> MKVQYCDSLVIGGGLAGLRAAVATQQKGLSTIVLSLIPVKRSHSAAAQGGMQASLGNSKMSDGDNEDLHFMDTVKGSDW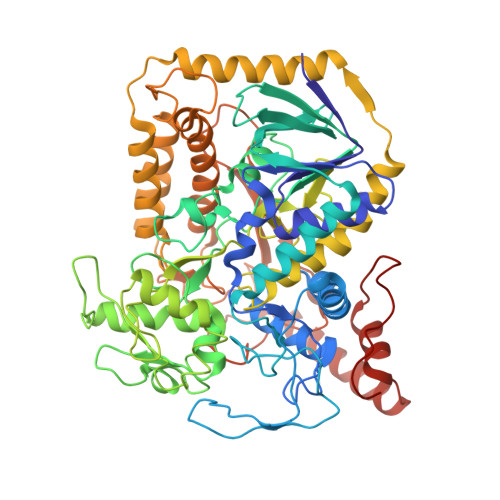GCDQKVARMFVNTAPKAIRELAAWGVPWTRIHKGDRMAIINAQKTTITEEDFRHGLIHSRDFGGTKKWRTCYTADATGHTMLFAVANECLKLGVSIQDRKEAIALIHQDGKCYGAVVRDLVTGDIIAYVAKGTLIATGGYGRIYKNTTNAVVCEGTGTAIALETGIAQLGNMEAVQFHPTPLFPSGILLTEGCRGDGGILRDVDGHRFMPDYEPEKKELASRDVVSRRMIEHIRKGKGVQSPYGQHLWLDISILGRKHIETNLRDVQEICEYFAGIDPAEKWAPVLPMQHYSMGGIRTDYRGEAKLKGLFSAGEAACWDMHGFNRLGGNSVSEAVVAGMIVGEYFAEHCANTQVDLETKTLEKFVKGQEAYMKSLVESKGTEDVFKIKNRMKDVMDDNVGIFRDGPHLEKAVKELEELYKKSKNVGIKNKRLHANPELEEAYRVPMMLKVALCVAKGALDRTESRGAHNREDYPKRDDINWLNRTLASWPNPEQTLPTLEYEALDVNEMEIAPGYRGYGAKGNYIENPLSVKRQEEIDKIQSELEAAGKDRHAIQEALMPYELPAKYKARNERLGDK> MGCSEKININEDKISHKIDIPDSAWTIGIGEKFKNAGHPNVKYPMIDDSYVQGAPLGGFGAGTIGRTYNGGFSRWHLEIGKNKYTTVYANQFSVFQKVEGNKDGVAQVLYAGEPENGYLSSWKWDYPKESGMYYALYPNSWYTYTNKDLPVQLAVKQFSPIIPYNYKETSYPVAVFKWTAYNPTNKNVDVSIMFTWQNMIGFFGKQVNVNSGNFNKIIKDKSKDSEIVAAVMGNISNDNEEWNGEYSIGVKKVPGVDISYKAKFVTTGDGSDLWHEFSKNGILDNKDDETPTKQDGIGSAIAVNFKLQPGQTIEVPFALSWDLPIMKFGGGDKWYKMYTKYFGKNGKNSFAILKEALNNYQKWEKMIDDWQKPILSNKSKPDWYKTALFNELYYLADGGTAWENGKVGEKDKRTNNMFGLLECFDYNYYETLDVRFYGSFPLVMLWPDIEKQVMRQFADTINVQDSSEFKVGSNGAMAVKKVQGMIPHDLGSSYALPWIKINAYDWQNPNIWKDLNSKYVLLVYRDYVLTGKTDKEFLKYTWKSVKTALDKLKEMDKDNDGIPDNEGIPDQTYDTWSMKGTSAYCGSLWLAALKAAQEIGKVLKDN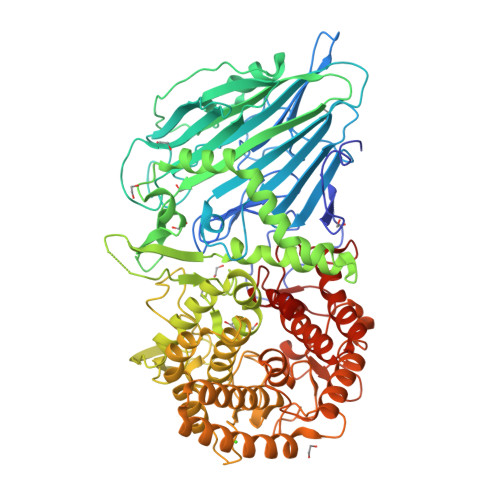EAYIKYNEWYKIAQQNFEKELWNGEYYNFDTESDHKDSIMADQLAGQWYADILRLGDILPKDHVQKALKKIYEFNVMKFENGKMGAVNGMRPDGIVDESDIQAQEVWTGVTYALASFMKYRGMTEEAYNTAYGVYKMTYDKSGKGYWFRTPEAWTKDGNYRASMYMRPLSIWSMEVNYNEV>MGSSHHHHHHHSSGLVPRGSHHMLEMQINLPEVHAEVTAQFVRYEKALTSNDTAVLNELFWNSPQTLRYGATENLYGYEAIAGFRATRSPNNLEKEIVRTVITTYGHDFATANIEFRRLSHSQLTGRQSQTWMRTSQ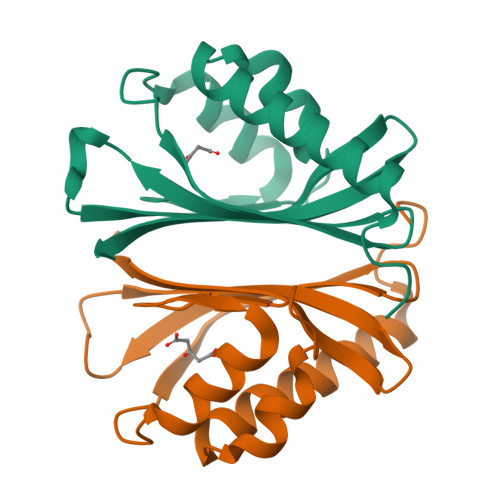GWRVVAAHVSLIALPVS[12x]> MLRWSRLLRGRPPPVMGHAKRMRFAGVDDNPSVTHKPWDTSEPLMADYGWERGKLPKFRARSPFHRQQIARRMVTELIRKDYVIVGGARAPALRILADHVVELAKAGDTDSRQQLAYFLHDPLMVDKAFDEYPRRFRDMNAKYAMMTRLKGRRRSDNVAMYFVEYKNRDMSDNHKGEDYTAGPERFFLPPRIIETEKGIQRPPHMQMAFDRWASKFKTEEFHHWWRLRHAKLRYWGVRNVPHPSDVDPLWTEKEEEEWHNEMLANTSDFEDFDLDDDSYEAAGEG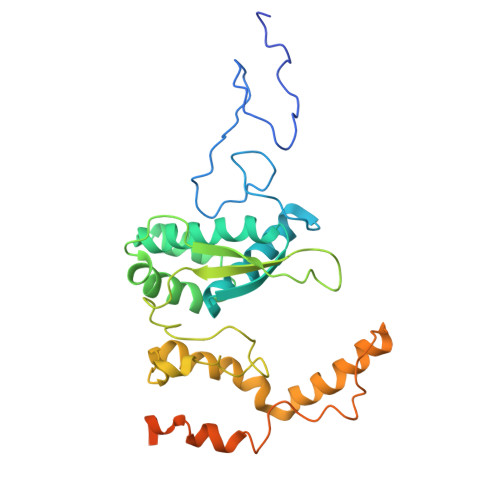GSQGGSSSLSGIGPEPQKKY> MNITKPFPLPTGYFDIPLGLAALSLAWFHLENLFPAARMVSDVLGIVASAVWILFILMYAYKLRYYFEEVRAEYHSPVRFSFIALIPITTMLVGDILYRWNPLIAEVLIWIGTIGQLLFSTLRVSELWQGGVFEQKSTHPSFYLPAVAANFTSASSLALLGYHDLGYLFFGAGMIAWIIFEPVLLQHLRISSLEPQFRATMGIVLAPAFVCVSAYLSINHGEVDTLAKILWGYG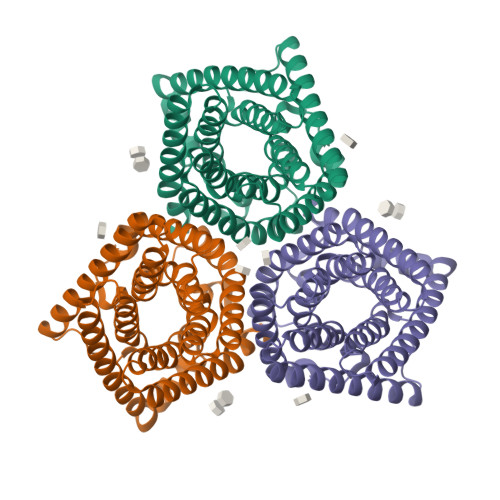FLQLFFLLRLFPWIVEKGLNIGLWAFSAGLASMANSATAFYHGNVLQGVSIFAFVFSNVMIGLLVLMTIYKLTKGQFFLK> MSKIVAVVVLAAFCVAMLVSDVSAKTSISVKGESNVDVVSQINSLVSSIVSGANVS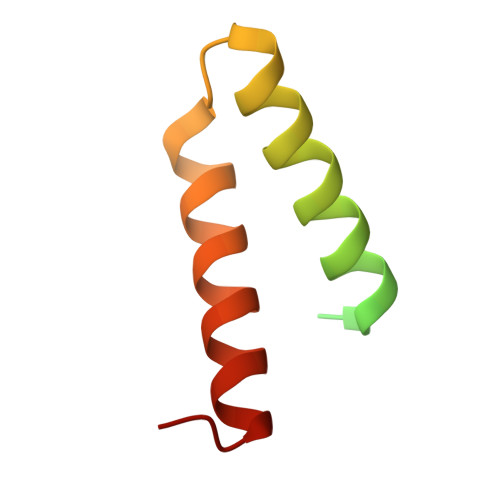AVLLAQTLVNILQILIDANVFA3-[2-[[5-[(4-ethenyl-3-methyl-5-oxidanylidene-pyrrol-2-yl)methyl]-3-(3-hydroxy-3-oxopropyl)-4-methyl-1~{H}-pyrrol-2-yl]methyl]-5-[[(3~{R},4~{R})-3-ethyl-4-methyl-5-oxidanylidene-3,4-dihydropyrrol-2-yl]methyl]-4-methyl-1~{H}-pyrrol-3-yl]propanoic 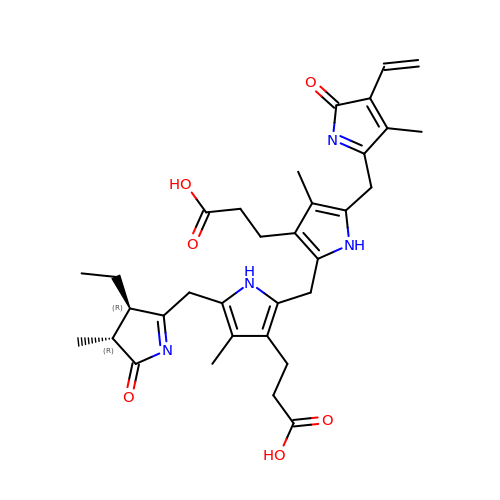acid | C33 H40 N4 O6 | FCSIENOPZMSJPT-WOJBJXKFSA-N>TRCTHLENRDFVTGVQGTTRVSLVLELGGCVTITAEGKPSIDVWLEDIFQESPAETREYCLHAKLSNTKVEARCPTTGPATLPEEHQANMVCKRDQSDRGWGNHCGFFGKGSIVACAKFECEEAKKAVGHVYDSTKITYVVKVEPHTGDYQAANETNENRKTAQFTVASEKVILDLGDYGDVSLTCKVASGIDVAQTVVMSLGSSKDHLPSAWQLHRDWFEDLALPWKHKDNQDWNSVEKLVEFGPPHAVKMDIFNLGDQTAVLLKSLAGVPLASVDNQKYHLKSGHVTCDVGLEKLKLKGTTYSMCDKTKFKWKRVPVDSGHDTVVMEVSYTGSDKPCRIPVRAVAHGVPTINVAMLITPNPTIETSGGGFIEMQLPPGDNIIYVGDLSQQWFQKGSTIGRMFEKTRKGLERLSVVGEHAWDFGSVGGILSSVGKAIHTVLGGAFNTLFGGVGFIPKMLLGVALVWLGLNARNPTMSMTFLAVGALTLMMTMG[3x];>[3x]SVVIPTHAQKDMVGRGHAWLKGDNIRDHVTRVEGWMWKNKLLTVAVVALAWLMLD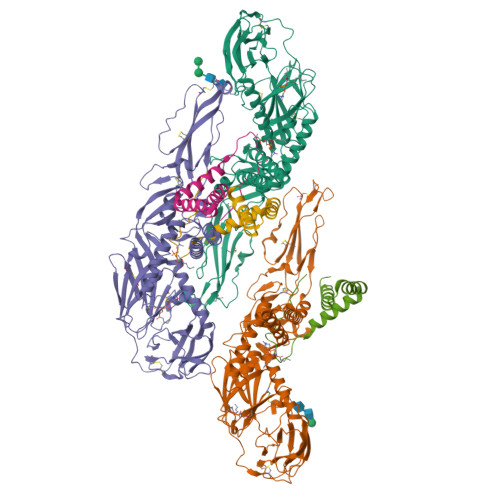SWMARVTVILLALSLGPVYA> MSMLKREDWYDLTRTTNWTPKYVTENELFPEEMSGARGISMEAWEKYDEPYKITYPEYVSIQREKDSGAYSIKAALERDGFVDRADPGWVSTMQLHFGAIALEEYAASTAEARMARFAKAPGNRNMATFGMMDENRHGQIQLYFPYANVKRSRKWDWAHKAIHTNEWAAIAARSFFDDMMMTRDSVAVSIMLTFAFETGFSNMQFLGLAADAAEAGDHTFASLISSIQTDESRHAQQGGPSLKILVENGKKDEAQQMVDVAIWRSWKLFSVLTGPIMDYYTPLESRNQSFKEFMLEWI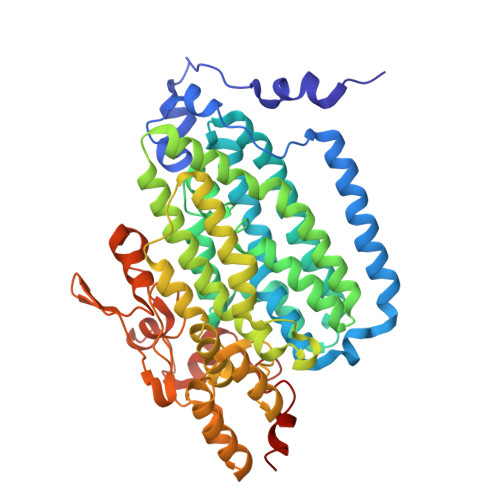VAQFERQLLDLGLDKPWYWDQFMQDLDETHHGMHLGVWYWRPTVWWDPAAGVSPEEREWLEEKYPGWNDTWGQCWDVITDNLVNGKPELTVPETLPTICNMCNLPIAHTPGNKWNVKDYQLEYEGRLYHFGSEADRWCFQIDPERYENHTNLVDRFLKGEIQPADLAGALMYMSLEPGVMGDDAHDYEWVKAYQKKTNAA>MLGSGFKAERLRVNLELVINRLKLLEEKKTELAQKARKEIADYLAAGKDERARIRVEHIIREDYLVEAMEILELYCDLLLARFGLIQSMKELDSGLAESVSTLIWAAPRLQSEVAELKIVADQLCAKYSKEYGKLCRTNQIGTVNDRLMHKLSVEAPPKILVERYLI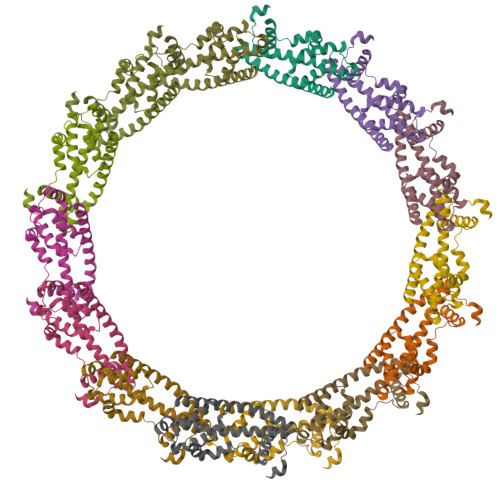EIAKNYNVPYEPDSVVMAEAPP[14x]>[8x]VKLAGNSSLCPINGWAVYSKDNSIRIGSKGDVFVIREPFISCSHLECRTFFLTQGALLNDKHSNGTVKDRSPHRTLMSCPVGEAPSPYNSRFESVAWSASACHDGTSWLTIGISGPDNGAVAVLKYN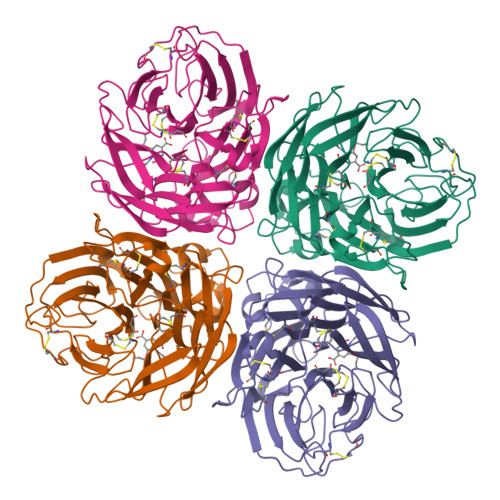GIITDTIKSWRNNILRTQESECACVNGSCFTVMTDGPSNGQASYKIFKMEKGKVVKSVELDAPNYHYEECSCYPNAGEITCVCRDSWHGSNRPWVSFNQNLEYQIGYICSGVFGDNPRPNDGTGSCGPVSSNGAYGVKGFSFKYGNGVWIGRTKSTNSRSGFEMIWDPNGWTETDSSFSVKQDIVAITDWSGYSGSFVQHPELTGLDCIRPCFWVELIRGRPKESTIWTSGSSISFCGVNSDTVGWSWPDGAELPFTI> ESEKI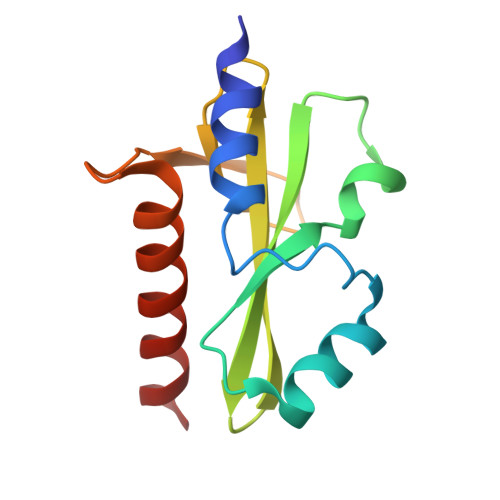YKVMEEIFVDRHYKENIRTGEEVKQYFSKSKAEFILRWSSANESDTENKYVFIAASFQASDGIHSIRYGINKNGELFSINTASNKVTPIDILPLGVMATLTQHITQNKELIEKAL> FPTIPLSRLFDNAMLRAHRLHQLAFDTYQEFEEAYIPKEQKYSFLQNPQTSLCFSESIPTPSNREETQQKSNLELLRISLLLIQSWLEPVQFLRSVFANSLVYGASDSNVYDLLKDLEEGIQTLMGRLEDGSPRTGQIFKQTYSKFDTNSHNDDALLKNYGLLYCFRKDMDKVETFLRIVQCRSVEGSCGF;>[2x]FSGSEATAAILSRAPWSLQSVNPGLKTNSSKEPKFTKCRSPERETFSCH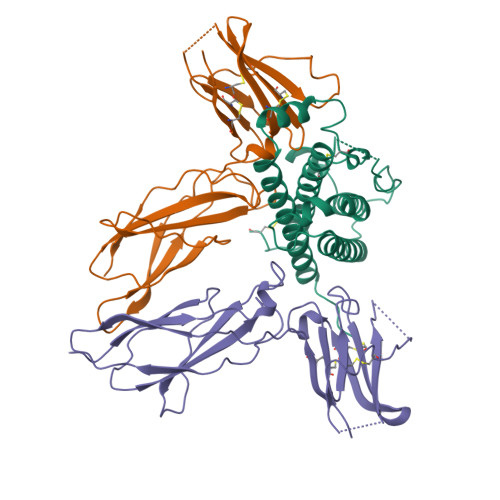WTDEVHHGTKNLGPIQLFYTRRNTQEWTQEWKECPDYVSAGENSCYFNSSFTSIWIPYCIKLTSNGGTVDEKCFSVDEIVQPDPPIALNWTLLNVSLTGIHADIQVRWEAPRNADIQKGWMVLEYELQYKEVNETKWKMMDPILTTSVPVYSLKVDKEYEVRVRSKQRNSGNYGEFSEVLYVTLPQMS> GYSLFPNSPKWTSKVVTYRIVSYTRDLPHITVDRLVSKALNMWGKEIPLHFRKVVWGTADIMIGFARGAHGDSYPFDGPGNTLAHAFAPGTGLGGDAHFDEDERWTDGSSLGINFLYAATHELGHSLGMGHSSDPNAVMYPTYGNGDPQNFKLSQDDIKGIQ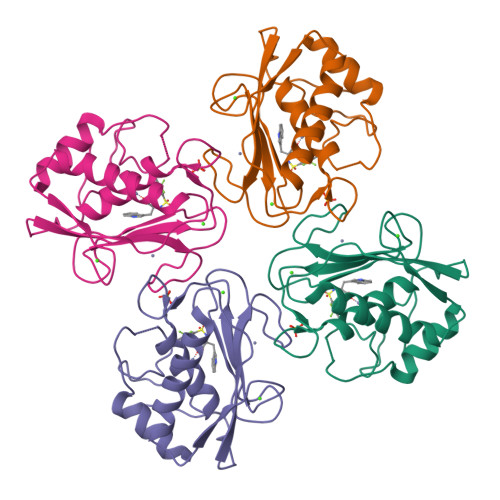KLY4-aminophenyl alpha-D-galactopyranoside | C12 H17 N O6 | 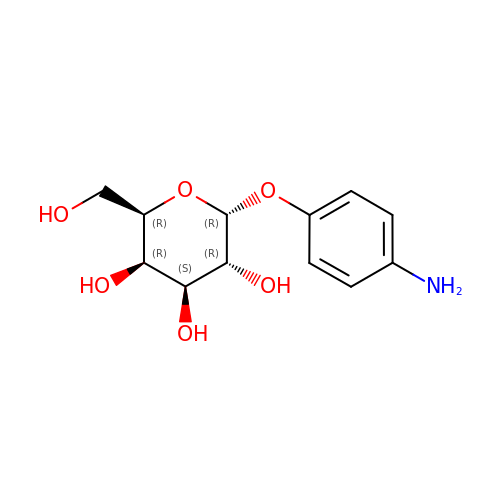MIAKOEWBCMPCQR-IIRVCBMXSA-N THYMIDINE-5'-DIPHOSPHO-BETA-D-XYLOSE | C15 H24 N2 O15 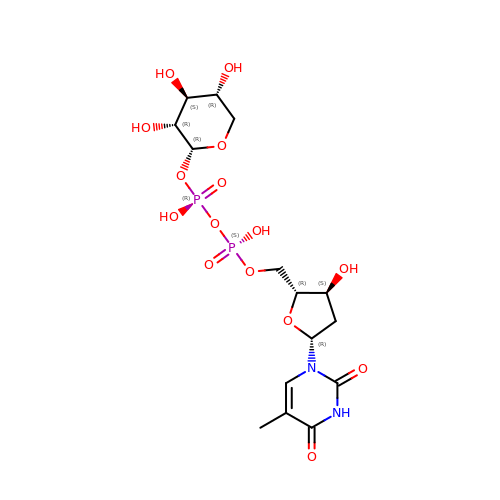P2 | AJUADKZRQSBUAK-KDGZBOQCSA-N> MGSNQSSSTSTKKLKAGNFDVAYQNPDKAIKGGNLKVAYQSDSPMKAQWLSGLSNDATFATMSGPGGGQDGLFFTDSGFKFIKGGAADVALDKESKTATITLRKDLKWSDGSEVTAKDYEFTYETIANPAYGSDRWTDSLANIVGLSDYHTGKAKTISGITFPDGENGKVIKVQFKEMKPGMTQSGNGY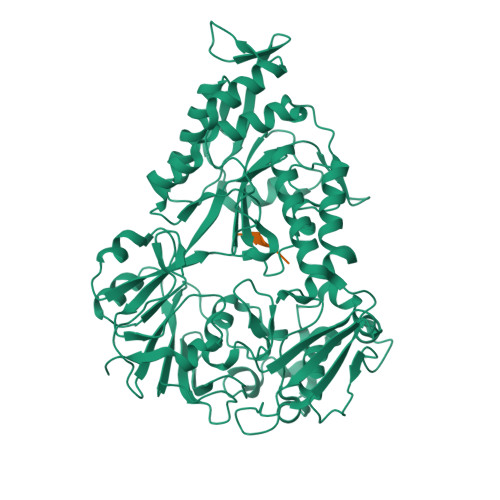FLETVAPYQYLKDVAPKDLASSPKTTTKPLVTGPFKPENVVAGESIKYVPNPYYWGEKPKLNSITYEVVSTAKSVAALSSSKYDIINGMVSSQYKQVKNLKGYKVLGQQAMYISLMYYNLGHYDAKNSINVQDRKTPLQDQNVRQAIGYARNVAEVDNKFSNGLSTPANSLIPPIFKQFTSSSVKGYEKQDLDKANKLLDEDGWKLNKSTGYREKDGKELSLVYAARVGDANAETIAQNYIQQWKKIGVKVSLYNGKLMEFNSWVDHMTTPPGANDWDITDGSWSLASEPSQQDLFSAAAPYNFGHFNDSEITKDLNDIDSAKSENPTYRKAAFVKYQEDMNKKAYVIPTNFMLNYTPVNKRVVGMTLDYGAMNTWSEIGVSSAKLATKGSIEGRHHHHHH;> AHAKA> SNAMENKLTEPLPTRMRILRAARQCFAENGFHSTSMKTICKASDMSPGTLYHHFPSKEALIEAIILEDQERALTHFREPLEGVGLVDYLVESTIAVTREDYAQRALVVEIMAEGMRNPQVAEMLTNKYHTIIASLVARFNDAQAKGEIGADVDKEMAARLLLATTYGVLS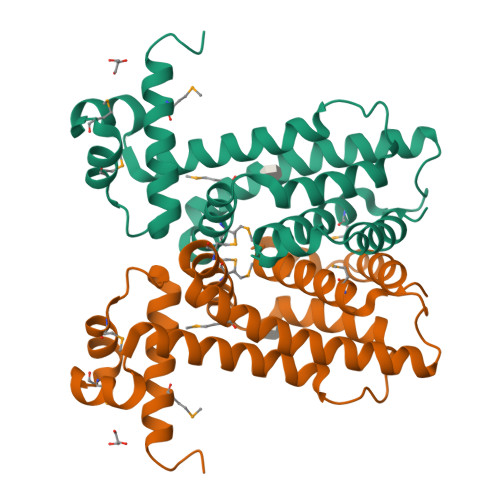DSSSAENARHVSFATTLRTMLTGLLKCNSAS>[2x]MMGSSHHHHHHHHHSSGENLYFQGGSMIEVTEVSIAELRDALESGRTTAVELVQAYLARIDA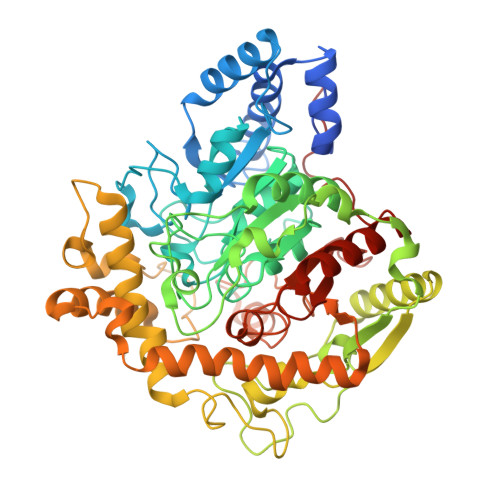YDAPGTPTALNAVVVRNPDALAEAQASDARRARGEPLGPLDGIPYTAKDSYLVKGLTAASGSPAFKDLVAQRDAFTVERLRAAGAICLGKTNMPPMANGGMQRGVYGRAESPYNAAYLTAPFASGSSNGAGTATAASFAAFGLAEETWSSGRGPASNNGLCAYTPSRGVISVRGNWPLTPTMDVVVPYARSMADLLEILDVVVADDPDTRGDLWRMQPWVPIPKASEVRPASYPALAAGAEALAGKRFGVPRMFINADPDAGTSESPGIGGPTGQRIHTRPSVIALWEQARKALEAAGAEVIEVDFPLVSNCEGDRPGAPTVFNRGLVSKEFLHDELWELSAWGFDDFLRANGDPKLNRLADVDGPQIFPHDPGTLPNREGDLAAGMDEYVRMAERGIKPWDRIATLPDGLRGLEETRRIDLEEWMRRLRLDAVLFPTVADVGPADADVNPASADIAWSNGVWVANGNLAIRHLGVPTVTVPMGVMADIGMPVGLTFAGRAYDDSALLRFAAAFESTGSRRIVPPRTPPLASK>[12x]ARHVA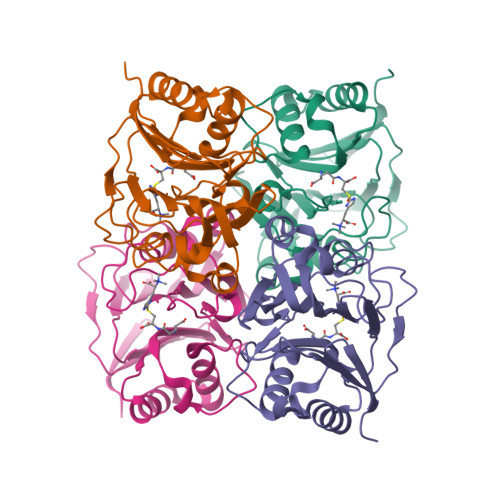WLGAPRSLADLVLDPPQGLLVQSYAPRRQKHGLMNADGWGAGFFDDDGVARRWRSDKPLWGDASFASVAPALRSRCVVAAVRSATIGMPIEPSASAPFSDGQWLLSHNGLVDRGVLPLTGAAESTVDSAILAALIFSRGLDALGATIAEVGELDPNARLNILAANGSRLLATTWGDTLSVLRRPDGVVLASEPYDDDPGWSDIPDRHLVDVRDAHVVVTPLLEHHHHHH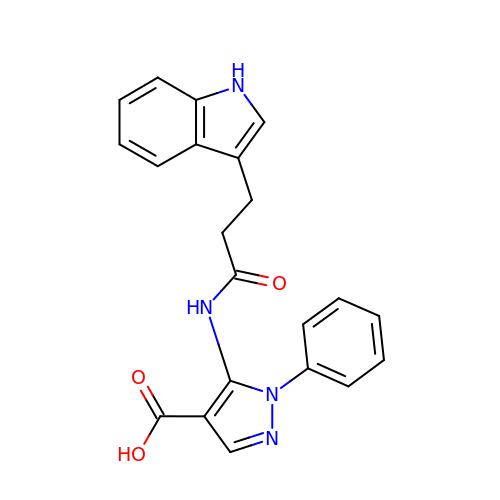5-{[3-(1H-indol-3-yl)propanoyl]amino}-1-phenyl-1H-pyrazole-4-carboxylic acid | C21 H18 N4 O3 | QMJGNSVNJWLCNN-UHFFFAOYSA-N> KEAIVFSQ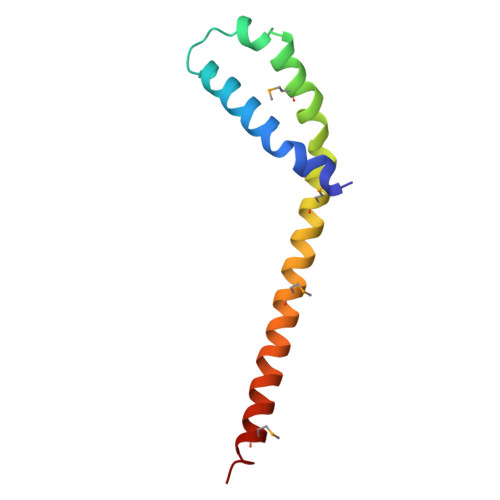KTTIDQLHNSLNAASKTGNSNEVLQDPHIGDMYGSVTPLRPQVTRMLGKYAKEKEDMLSLRQVLANAERSYNQLMDRAAN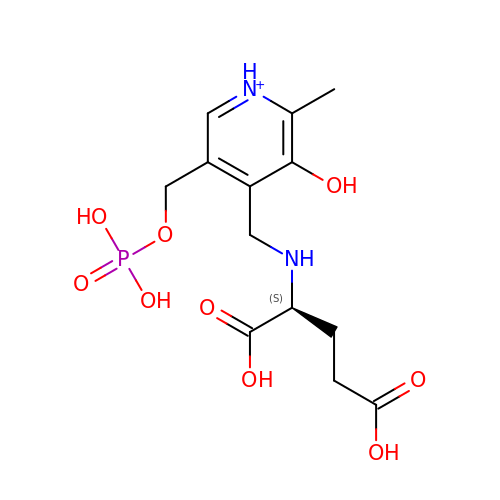4-[(1,3-DICARBOXY-PROPYLAMINO)-METHYL]-3-HYDROXY-2-METHYL-5-PHOSPHONOOXYMETHYL-PYRIDINIUM | C13 H20 N2 O9 P | JMRKOGDJNHPMHS-JTQLQIEISA-O> GSHMGGRLEGLTQDLRQLQESEQQLDHLMNICTTQLRLLSEDTDSQRLAYVTCQDLRSIADPAEQMVMVIKAPPETQLQAVDSSENFQISLKSKQGPIDVFL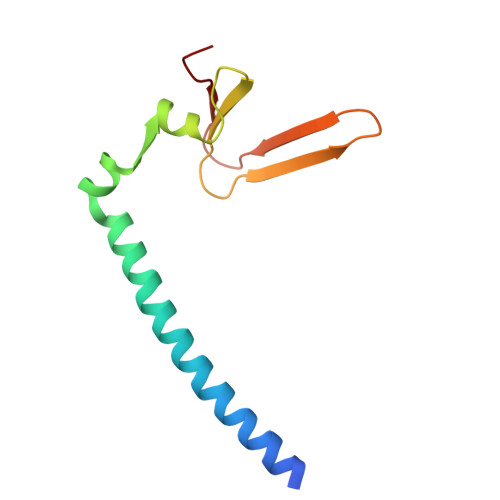CPEE Type 2 promoters contain two gene-internal DNA-binding elements named A- and B-box that are recognized by the general transcription factor IIIC (TFIIIC). TFIIIC is a six-subunit protein complex of ∼0.5 MDa mass consisting of two subcomplexes of similar size, τA and τB, which contact A-box and B-box promoter elements, respectively. We therefore structurally characterized the S. pombe TFIIIC Sfc1/Sfc7 subcomplex and present crystal structures of two structural modules. The N-terminal moiety of Sfc1 (Sfc1-NT) and subunit Sfc7 heterodimerize through a triple β-barrel fold most similar to the dimerization domains of general transcription factor TFIIF Rap30/Rap74, whereas the C-terminal DNA-binding domain of Sfc1 (Sfc1-DBD) comprises a winged-helix domain most similar to the winged-helix domain present in TFIIF Rap30 that is packed against a second domain with novel fold.

The crystal structure of the C-terminal domain of Sfc1 (Sfc1-DBD, residues 186–396) was solved at 1.45 Å resolution by MAD using selenomethionine-substituted protein. The Sfc1-DBD structure forms a compact domain that can be further divided into two subdomains. The first domain (residues 186–283) adopts a winged-helix domain fold with canonical α1 -β1-α2-α3-β2-β3 topology. The third helix α3 is not continuous, but split into two short helices α3a and α3b. The second domain (residues 284–396) consists of five α-helices and two β-strands and adopts a novel fold with no significant similarity to any known structure. Subsequently, we will refer to this domain as winged-helix-interacting (WHI) domain. Structural comparison using program DALI identifies the winged-helix domain of Rap30 (29) as the structure with the closest similarity to the winged-helix domain of Sfc1 (Z-score = 6.1, rmsd61CA = 2.7 Å) among the many winged-helix domains present in the PDB database. Inspection of the Sfc1-DBD electrostatic surface potential identifies an extended basic region on one side of the Sfc1-DBD that could interact with DNA, whereas the opposite side appears rather uncharged. The basic interaction surface of Sfc1-DBD shows two separate positively charged patches. One continuous larger patch runs diagonally across the surface of Sfc1-DBD and predominantly comprises basic residues of helices α2 and α3 of the winged-helix domain.

> GAMGKGQCRVWIITTNMGVESVPTCRHSKLGEPSKTIQEVIEALKPLFEKRPVWTRRALLNHLDPSYTHYLKFALPYLSYLWTSGPFRDTYTRFGYDPRKDSNAAAYQALFFKLKLNGKHKGTKTHVFDGKTLFPTNRVYQVCDIVDPTIAPLLKDTQLRSECHRDTGWYRSGRYYKVRDLMREKLFALIEGEMPSEVAVNMILNAEEVEESDRY> NNIDFDSIAKMLLIKYKDFILSKFKKAAPVENIRFQNLVHTNQFAQGVLGQSQHLCTVYDNPSWHSIVLETLDLDLIYKNVDKEFAKDGHAEGENIYTDYLVKELLRYFKQDFFKWCNKPDCNHCGQNTSENMTPLGSQGPNGEESKFNCGTVEIYKCNRCGNITRFPRYNDPIKLLETRKGRCGEWCNLFTLILKSFGLDVRYVWNREDHVWCEYFSNFLNRWVHVDSCEQSFDQPYIYSINWNKKMSYCIAFGKDGVVDVSKRYILQNELPRDQIKEEDLKFLCQFITKRLRYSLNDDEIYQLACRDEQEQIELIRGKTQETKSESVSAASKS;> G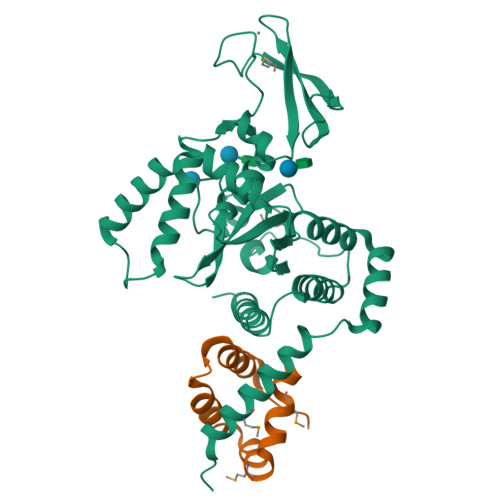TTGGATDAAQGGPPGSIGLTVEDLLSLRQVVSGNPEALAPLLENISARYPQLREHIMANPEVFVSMLLEAV> MTDALEQSVLALEGTVSVLKDSVESLKCANEPSTNLASTMLQTKRVFRLVPEYDVERSKLDLIEEVEPLVRTLGDKLRKSMGRMQRELDTLQQTYELNDLRLKKNISMDDDDALNSPDMGQEYEGRDADDVVMMA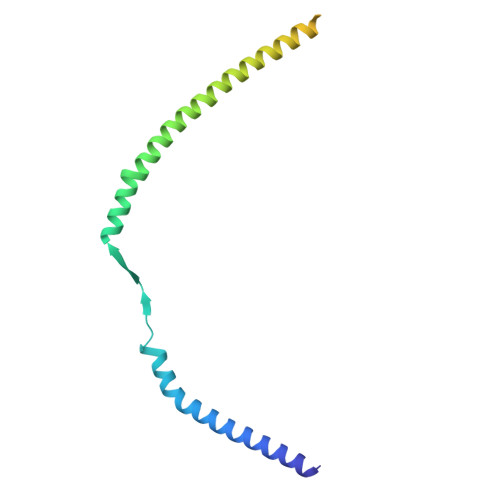SSTNEELEELKKLKEKKKQLENKLEILKQK>MFQRSIPALITPFTKDNLIDEDSFVDHIEWQISEGSSGLVPAGTTGESSTLSYEEHCRVVELCVKTAAGRVPVMAGAGSNNTKESIELAQYAQNTGADALLVVVPYYNKPNKKGLLAHFGSIANAVSLPIYIYNNPSRTVIEMDVDTMAELVKTYSNIVGVKDATGRIELASGQRIACGSDFIQLSGDDSSALGFNVHGGVGCISVTANVAPRICAEFQKAISEGDYRQALEYQDKLFPLHQALFIEPSISSVKYALSRLGRNVSLVVRAPMVS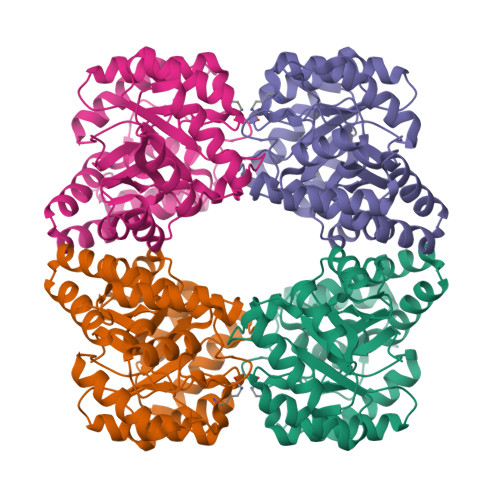ILEKETMFAIDQALDHIGLCAGHHHHHH[6x]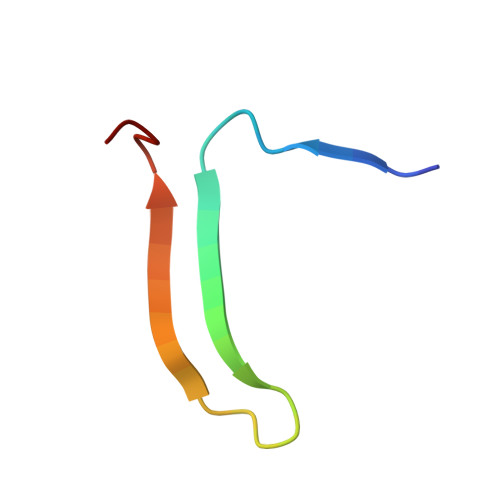> YPQVIVDHPFLYLIRNRKSGIILFMGRVMNPHH> MIAQGQTLPNATLSQLTKEGMVHHPVLELFAGKKVVLFAVPGAFTPTDSEAHLPGYIVLADQLKAKGVDLIASVSVNDAFVMKAWGEAQNAEEILMLADGDASFTKALGLEMDTAGFGGLRSQRYAMIIDNGVVTTLNVEAPKSFEVSNAETILAALEHHHHHH

V. vulnificus Prx3 (VvPrx3) belongs to the 1-Cys class of Prxs, with one conserved catalytic cysteine (Cys48), and has been shown to be involved in pathogenicity in a mouse model. Cys48 is the CP residue that is crucial for the function of the protein. All three crystal structures of VvPrx3 revealed a protomer exhibiting a compact and spherical structure without a C-terminal extension region, similar to the previously reported 1-Cys Prx AhpE from Mycobacterium tuberculosis (Li et al., 2005). All three crystal structures of VvPrx3 [reduced Prx3 (C48D/C73S), oxidized Prx3 (C73S) and H2O2-bound Prx3 (C48D/C73S)] showed a similar dimeric assembly in the crystals characterized by an A-type dimeric interface, similar to that in AhpE from M. tuberculosis (Li et al., 2005).

To study the structure of Prx3 in the reduced state, crystals of a VvPrx3 (C48D/C73S) variant were also obtained. The CP Cys48 in VvPrx3 was replaced with a non-oxidizable Asp residue, which could also partly mimic an over-oxidized form (Cys-SO2H) of VvPrx3. The crystal belonged to a different space group, P3221, and the VvPrx3 (C48D/C73S) structure [named reduced Prx (C48D/C73S) in this study] was determined by the molecular replacement approach. The crystal structure representing the reduced Prx3 showed a typical dimeric interface, called the A-type interface.> GEPLYTEQDLAVNGREGFPNYRIPALTVTPDGDLLASYDGRPTGIGAPGPNSILQRRSTDGGRTWGEQQVVSAGQTTAPIKGFSDPSYLVDRETGTIFNFHVYSQRQGFAGSRPGTDPADPNVLHANVATSTDGGLTWSHRTITADITPDPGWRSRFAASGEGIQLRYGPHAGRLIQQYTIINAAGAFQAVSVYSDDHGRTWRAGEAVGVGMDENKTVELSDGRVLLNSRDSARSGYRKVAVSTDGGHSYGP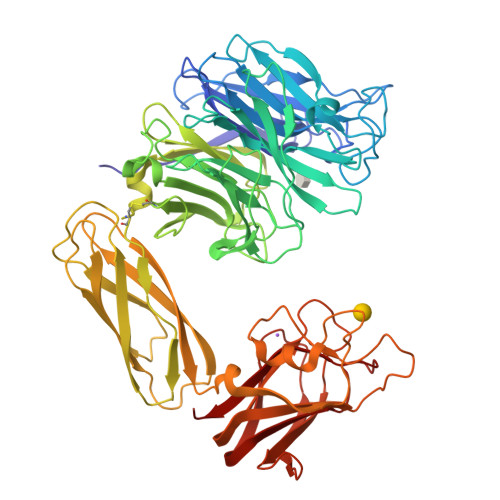VTIDRDLPDPTNNASIIRAFPDAPAGSARAKVLLFSNAASQTSRSQGTIRMSCDDGQTWPVSKVFQPGSMSYSTLTALPDGTYGLLYEPGTGIRYANFNLAWLGGICAPFTIPDVALEPGQQVTVPVAVTNQSGIAVPKPSLQLDASPDWQVQGSVEPLMPGRQAKGQVTITVPAGTTPGRYRVGATLRTSAGNASTTFTVTVGLLDQARMSIADVDSEETAREDGRASNVIDGNPSTFWHTEWSRADAPGYPHRISLDLGGTHTISGLQYTRRQNSANEQVADYEIYTSLNGTTWDGPVASGRFTTSLAPQRAVFPARDARYIRLVALSEQTGHKYAAVAELEVEGQR> GDTETAIDNAIARVADTVASGPSNSTSIPALTAVETGHTSQVEPSDTMQTRHVKNYHSRSESTVENFLSRSACVYIEEYYTKDQDNVNRYMSWTINARRMVQLRRKFELFTYMRFDMEITFVITSRQLPGTSIAQDMPPLTHQIMYIPPGGPVPNSVTDFAWQTSTNPSIFWTEGNAPPRMSIPFISIGNAYSNFYDGWSHFSQNGVYGYNALNNMGKLYARHVNKDTPYQMSSTIRVYFKPKHIRVWVPRPPRLSPYIKSSNVNFNPTNLTDERSSI;> GYSDRVRSLTLGNSTITTQESANVVVGYGRWPEYLRDDEATAEDQPTQPDVATCRFYTLESVQWEKNSAGWWWKFPEALKDMGLFGQNMLYHYLGRAGYTIHVQCNASKFHQGCLLVVCVPEAEMGCSQTDKEVAAMNLTKGEAAHKFEPTKTTGEHTVQSIVCNAGMGVGVGNLTIYPHQWINLRTNNCATIVMPYVNSVPMDNMFRHYNFTLMVIPFAPLDYAAQASEYVPVTVTIAPMCAEYNGLRLAYQQ;> GFPVLNTPGSNQFMTSDDFQSPSAMPQFDVTPHMDIPGEVHNLMEIAEVDSVVPVNNIKVNLQSMDAYHIEVNTGNHQGEKIFAFQMQPGLESVFKRTLMGEILNYYAHWSGSIKLTFTFCGSAMATGKLLLAYSPPGADVPATRKQAMLGTHMIWDIGLQSSCVLCIPWISQTHYRLVQQDEYTSAGNVTCWYQTGIVVPPGTPNKCVVLCFASACNDFSVRMLRDTPFIGQTALLQ;> DCGLPPDVPNAQPALEGRTSFPEDTVITYKCEESFVKIPGEKDSVICLKGSQWSDIEEFCNRSCEVPTRLNSASLKQPYITQNYFPVGTVVEYECRPGYRREPSLSPKLTCLQNLKWSTAVEFCKKKSCPNPGEIRNGQIDVPGGILFGATISFSCNTGYKLFGSTSSFCLISGSSVQWSDPLPECREIYCPAPPQIDNGIIQGERDHYGYRQSVTYACNKGFTMI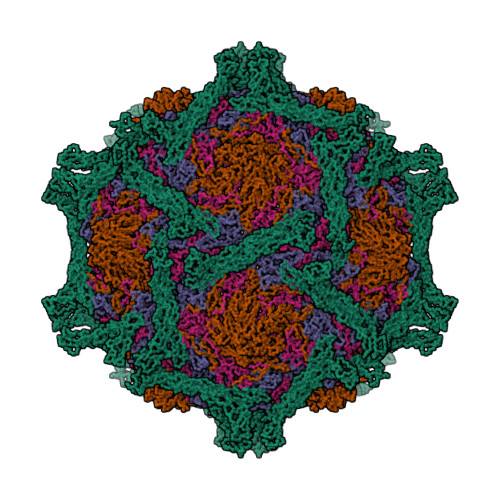GEHSIYCTVNNDEGEWS>[30x]MANPTLFVSYDQNGKKLSFANWISVLSPQDTPFVSMTGKESINQTIFSWQTDALASVDGNNAHVEGSRAEDGEMKPTVIKSNVTQILRKVVRVSDTANTTANYGRGRELMYQLEKKGKEIKRDLEKILLSGQARTDVLADQYLTNSAADPAVAGLNDTHAARKTGAFQFLCAHGGLAGGVVDKTKNGPADPDTGAVTVKVAQNASNPTTNIGFDEADIFDMTLQLYTAGSEADIIMINPAHAKIFAGLQENTQGSRKRIFENTKQFIYEVNSITDPLGQSYKIIVNRWMPTDAVYFFRSADWTQMVLRAPKRTELAKDGSYEKWMIEMEVGLRHRNPYASGVLFTAAGKAAA

Escherichia coli phage SU10 belongs to the genus Kuravirus from the class Caudoviricetes of phages with short non-contractile tails. Here we show that the virion of SU10 has a prolate head, containing genome and ejection proteins, and a tail, which is formed of portal, adaptor, nozzle, and tail needle proteins and decorated with long and short fibers. In contrast to other short-tailed phages, the tails of Kuraviruses elongate upon cell attachment. After binding to the host, SU10 tail, nozzle proteins, and short fibers re-arrange to form a nozzle that extends the tail.

The capsid is closed on both ends with caps formed by the major capsid proteins organized with local T = 4 quasi-icosahedral symmetry. The closure of the caps is enabled by pentamers, which are bent in contrast to the flatter hexamers. The hexamers in the caps are more bent (H4, H5; 149-150°), whereas those that form the tubular part of the capsid are relatively flat (H1, H2L, H2R, H3; 154–164°). The major difference between the capsid proteins forming hexamers and pentamers is in the structure of the annular loop positioned at the tip of the axial domain. In hexamers, the annular loop protrudes away from the axial domain. In contrast, in subunits forming pentamers the annular loop is bent 90° towards the capsid center. The beta-strands from the loops of major capsid proteins from a pentamer form a beta-barrel with a central pore with a diameter of 8 Å that penetrates through the capsid. The pore may serve for the passage of ions and water molecules from and into the capsid during genome packaging and ejection. The DNA strands from the outermost layer of the genome curve to avoid the beta-barrels protruding from pentamers of capsid proteins.>[6x]MADHSASGAPALSTNIESGKFDEKAAEAAAYQPKPKVEDDEDEDIDALIEDLESHDGHDAEEEEEEATPGGGRVVPEDMLQTDTRVGLTSEEVVQRRRKYGLNQMKEEKENHFLKFLGFFVGPIQFVMEGAAVLAAGLEDWVDFGVICGLLLLNAVVGFVQEFQAGSIVDELKKTLALKAVVLRDGTLKEIEAPEVVPGDILQVEEGTIIPADGRIVTDDAFLQVD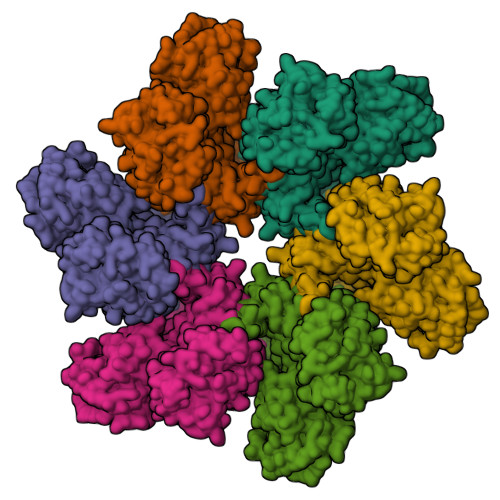QSALTGESLAVDKHKGDQVFASSAVKRGEAFVVITATGDNTFVGRAAALVNAASGGSGHFTEVLNGIGTILLILVIFTLLIVWVSSFYRSNPIVQILEFTLAITIIGVPVGLPAVVTTTMAVGAAYLAKKKAIVQKLSAIESLAGVEILCSDKTGTLTKNKLSLHDPYTVAGVDPEDLMLTACLAASRKKKGIDAIDKAFLKSLKYYPRAKSVLSKYKVLQFHPFDPVSKKVVAVVESPQGERITCVKGAPLFVLKTVEEDHPIPEEVDQAYKNKVAEFATRGFRSLGVARKRGEGSWEILGIMPCMDPPRHDTYKTVCEAKTLGLSIKMLTGDAVGIARETSRQLGLGTNIYNAERLGLGGGGDMPGSEVYDFVEAADGFAEVFPQHKYNVVEILQQRGYLVAMTGDGVNDAPSLKKADTGIAVEGSSDAARSAADIVFLAPGLGAIIDALKTSRQIFHRMYAYVVYRIALSIHLEIFLGLWIAILNRSLNIELVVFIAIFADVATLAIAYDNAPYSQTPVKWNLPKLWGMSVLLGVVLAVGTWITVTTMYAQGENGGIVQNFGNMDEVLFLQISLTENWLIFITRANGPFWSSIPSWQLSGAIFLVDILATCFTIWGWFEHSDTSIVAVVRIWIFSFGIFCIMGGVYYILQDSVGFDNLMHGKSPKGNQKQRSLEDFVVSLQRVSTQHEKSQ>[2x]GMNGREVAHRPLRKDAERNRKRVIAAARELFAVHGLESTLNEVAHHAGLG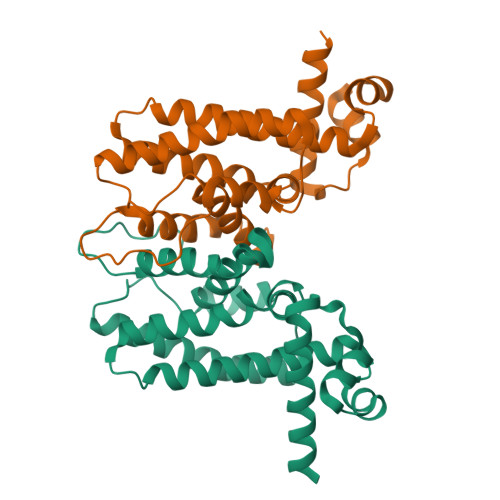VGTVYRRFPTKEALFEAIYVDGMDQLSGLAEAALRHENSWEGFEWFVHQMCEITATNRGLREIAFSKAHGGDHVEAGRARLLPLLSKVVERAQEDGYLRPEASATDMPFFGVLTGAVSEFAGEVNADLWRRYMAILIEGMRRRDDQERLEVDALDEAQIDAAMTTWQPAGSG>KPFTVPILTVEEMSNSRFPIPLEKLYTGPSSAFVVQPQNGRCTTDGVLLGTTQLSAVNICNFRGDVTRVGISHDYTMNLVSQNWNNYDPTEEIPAPLGTPDFVGKIQGLLTQTTRADGSTRAHKATVSTGSVHFTPKLGSVQFTTDTNNDFQTGQNTKFTPVGVIQDGDHHQNEPQQWVLPNYSGTSGHNVHLAPAVAPTFPGEQLLFFRSTMPGCSGYPNMNLDCLLPQEWVSHFYQEAAPAQSDVALLRFVNPDTGRVLFECKLHK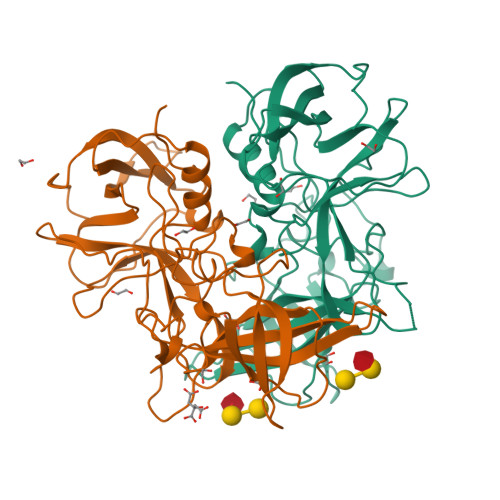SGYITVAHTGPYDLVIPPNGYFRFDSWVNQFYTLAPM[2x]>[2x]GPLGSMSGIALSRLAQERKAWRKDHPFGFVAVPTKNPDGTMNLMNWECAIPGKKGTPWEGGLFKLRMLFKDDYP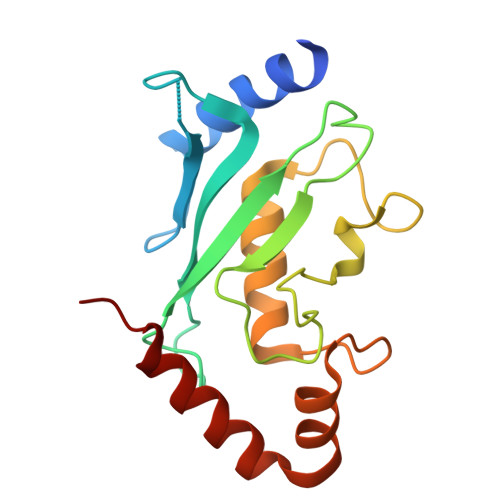SSPPKCKFEPPLFHPNVYPSGTVCLSILEEDKDWRPAITIKQILLGIQELLNEPNIQDPAQAEAYTIYCQNRVEYEKRVRAQAKKFAPS;>GPLGSQELRLRVQGKEKHQMLEISLSPDSPLKVLMSHYEEAMGLSGHKLSFFFDGTKLSGKELPADLGLESGDLIEVWG[2x]Toll-like Receptor 3 (TLR3) plays a key role in anti-viral defenses by inducing a potent immune response against double-stranded RNAs (dsRNAs) produced by viral infection. Previous crystallographic studies show that RNA ligand binds to the extracellular domains of TLR3 and induces the formation of a homodimer of TLR326. The charge interaction with the phosphate backbone of the RNA double helix plays the principal role in the interaction. The ligand-binding site involves both the N and C-terminal parts of the TLR3 ectodomain.

The closest contact area between the dimeric TLR3 units is composed of the negatively charged N-terminal and the positively charged C-terminal residues of the neighboring ectoTLR3 dimers. To test their role in TLR3 clustering, we made two charge-reversion mutations. The N-terminal mutant, NT-mut had a triple mutation of K117D, K139D and K145D and the C-terminal mutant, CT-mut had a triple mutation of D523K, D524K and E527K of ectoTLR3. For the cryo-EM study, the mutant ectoTLR3 domains were produced and mixed with poly(I:C). The micrographs of the resulting complexes show that the clustering of ectoTLR3 is significantly reduced or entirely blocked by the mutations. The dimeric structure of the mutant ectoTLR3 is still superimposable with that of the wild-type ectoTLR3. Therefore, the effect of the mutation is not due to a conformational change of the TLR3 nor the blocking of TLR3 dimerization. The TLR3-RNA interaction alone cannot explain the “ordered” clustering because the entropic effect will randomly distribute the bound TLR3 dimers along the dsRNA strands. The long-range charge interaction between the ectodomains of the TLR3 dimers contributes to clustering as shown in Fig. 5.

>[2x]ADPKCTVSHEVADCSHLKLTQVPDDLPTNITVLNLTHNQLRRLPAANFTRYSQLTSLDVGFNTISKLEPELCQKLPMLKVLNLQHNELSQLSDKTFAFCTNLTELHLMSNSIQKIKNNPFVKQKNLITLDLSHNGLSSTKLGTQVQLENLQELLLSNNKIQALKSEELDIFANSSLKKLELSSNQIKEFSPGCFHAIGRLFGLFLNNVQLGPSLTEKLCLELANTSIRNLSLSNSQLSTTSNTTFLGLKWTNLTMLDLSYNNLNVVGNDSFAWLPQLEYFFLEYNNIQHLFSHSLHGLFNVRYLNLKRSFTKQSISLASLPKIDDFSFQWLKCLEHLNMEDNDIPGIKSNMFTGLINLKYLSLSNSFTSLRTLTNETFVSLAHSPLHILNLTKNKISKIESDAFSWLGHLEVLDLGLNEIGQELTGQEWRGLENIFEIYLSYNKYLQLTRNSFALVPSLQRLMLRRVALKNVDSSPSPFQPLRNLTILDLSNNNIANINKKMLKGLEKLEILDLQHNNLARLWKHANPGGPIYFLKGLSHLHILNLESNGFDEIPVEVFKDLFELKIIDLGLNNLNTLPASVFNNQVSLKSLNLQKNLITSVEKKVFGPAFRNLTELDMRFNPFDCTCESIAWFVNWINETHTNIPELSSHYLCNTPPHYHGFPVRLFDTSSCKHHHHHH> MIKVEIKPSQAQFTTRS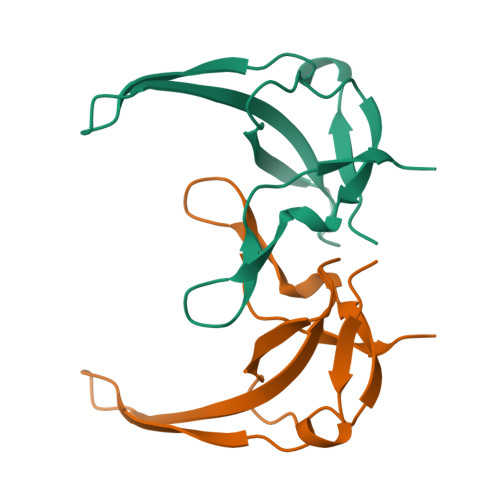GVSRQGKPYSLNEQLCYVDLGNEYPVLVKITLDEGQPAYAPGLYTVHLSSFKVGQFGSLMIDRLRLVPAK> SLDNNFYSVEIGDSTFTVLKRY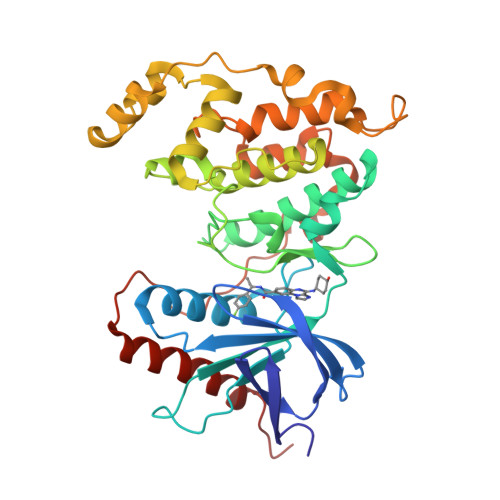QNLKPIGSGAQGIVCAAYDAILERNVAIKKLSRPFQNQTHAKRAYRELVLMKCVNHKNIIGLLNVFTPQKSLEEFQDVYIVMELMDANLCQVIQMELDHERMSYLLYQMLCGIKHLHSAGIIHRDLKPSNIVVKSDCTLKILDFGLARTAGTSFMMTPYVVTRYYRAPEVILGMGYKENVDLWSVGCIMGEMVCHKILFPGRDYIDQWNKVIEQLGTPCPEFMKKLQPTVRTYVENRPKYAGYSFEKLFPDVLFPADSEHNKLKASQARDLLSKMLVIDASKRISVDEALQHPYINVWYDPSEAEAPPPKIPDKQLDEREHTIEEWKELIYKEVMDWRKGIITIT Npro is a key effector protein of pestiviruses such as bovine viral diarrhea virus and abolishes host cell antiviral defense mechanisms. The nonstructural protein Npro (N-terminal protease) is the very first protein to be synthesized, releasing itself from the nascent polypeptide chain via a single, autoproteolytic cleavage event (Wiskerchen et al., 1991). Detached Npro is proteolytically inactive but acts as a viral immediate effector to modulate the host cell’s antiviral defenses (Ruggli et al., 2003). The overall structure revealed two compacted folding units: a protease domain (orange) and an interaction domain (I-domain, green).

Here, we present crystal structures of Δ(2–21)Npro from a BVDV-3/HoBi-like strain to 1.25 Å resolution, revealing a two-domain structure. We determined 1.25 Å and 1.5 Å crystal structures for solubly expressed and in-vitro-folded Npro, respectively. In neither case could we observe zinc binding at the TRASH motif but disulfide bridging between Cys112 and Cys134. The mixed disulfide of the third cysteine 138 with the reducing agent 1-thioglycerol present in the protein buffer indicated oxidizing conditions during crystal growth. Individual C112A, C134A, C138A, as well as D136N mutations in the TRASH motif abolished its zinc coordination and partially interrupted IRF3/IRF7 interactions in the Npro homologs Alfort and BVDV-1 (Fiebach et al., 2011; Ruggli et al., 2009; Szymanski et al., 2009). These findings corroborate our modeling studies, indicating that TRASH disulfides are reversible and able to adopt a zinc binding conformation without major alterations. The unexpected disulfide may point to such a function in Npro that awaits further investigation.

> MEPLYDKNGAVLFGEPSDTHPQSTLKLPHPRGEKEVIVGIRDLPRKGDCRTGNRLGPVSGLFVKPGPVFYQDYSGPVYHRAPLEQFKQAPMCEVTKRIGRVTGSDGNLYHMYVCTDGCILVKTAKHHHHHVLKWVYNVLDSPIWVTSC>[2x]SLAPYASLTEIEHLVQSVCKSYRETCQLRLEDLLRQRSNIFSREEVTGYQRKSMW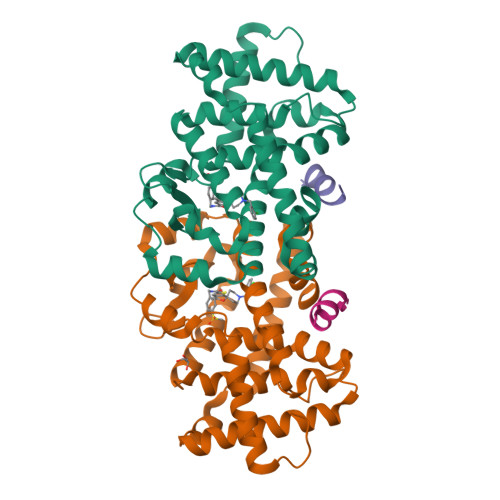EMWERCAHHLTEAIQYVVEFAKRLSGFMELCQNDQIVLLKAGAMEVVLVRMCRAYNADNRTVFFEGKYGGMELFRALGCSELISSIFDFSHSLSALHFSEDEIALYTALVLINAHRPGLQEKRKVEQLQYNLELAFHHHLCKTHRQSILAKLPPKGKLRSLCSQHVERLQIFQHLHPIVVQAAFPPLYKELFS;>[2x]EKHKILHRLLQDS> GHG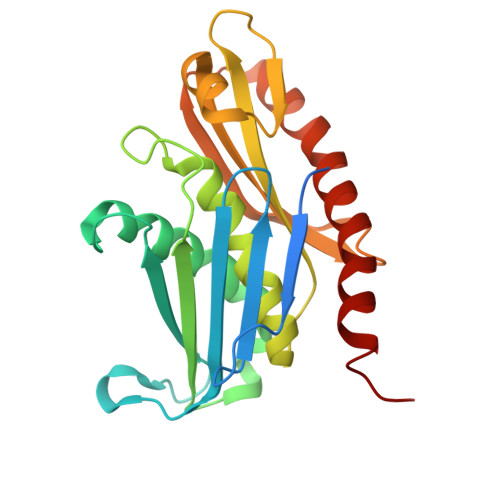NNKEPNTKNRLDSAEKKKKMSVQAEIGILDHVDGSSEFVSQDTKVICSVTGPIEPKARQELPTQLALEIIVRPAKGVATTREKVLEDKLRAVLTPLITRHCYPRQLCQITCQILESGEDEAEFSLRELSCCINAAFLALVDAGIALNSMCASIPIAIIKDTSDIIVDPTAEQLKISLSVHTLALEFVNGGKVVKNVLLLDSNGDFNEDQLFSLLELGEQKCQELVTNIRRIIQDNISPRLVV> GSHMDSTTIQQNKDTLSQIVVFPTGNYDKNEANAMVNRLANIDGKYLNALKQNNLKIKLLSGKLTDEKEYAYLKGVVPKGWEGTGKTWDDVPGLGGSTVALRIGFSNKGKGHDAINLELHATAHA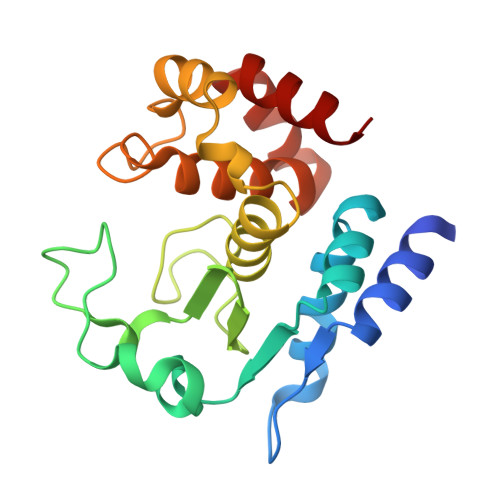IDHIVLNDISKSAQFKQIFAKEGRSLGNVNFLGVYPAEFFAESFAYYYLNQDTNSKLKSACPQTYSFLQNLAK>MSRLDKSKVINSALELLNEVGIEGLTTRKLAQKLGVEQPTLYWHVKNKRALLDALAIEMLDRHHTHFSPLEGESWQDFLRNNAKSFRNALLSHRDGAKVHLGTRPTEKQYETLENQLAFLTQQGFSLENALYALSAVGHFTLGSVLEDQEHQVAKEERETPTTDSMPPLLRQAIELFDHQGAEPAFLHGLESLIRGFEVQLTALLQIV[4x];>XWTWNAYAFAAPSG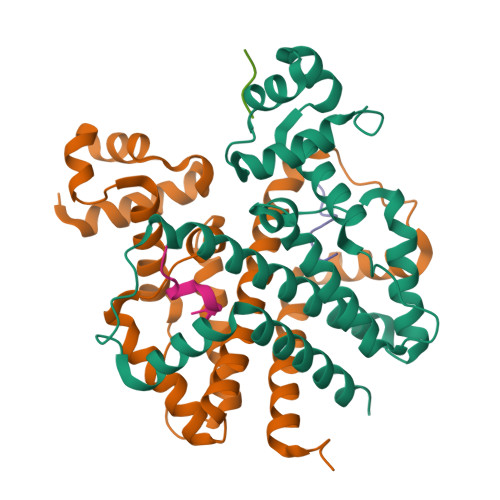GGS[5x]> MLTSSSHHGRSYDVFLSFRGEDTRKTFVGHLFNALIEKGIHTFMDDKELKRGKSISSELMKAIGESRFAVVVFSKNYASSTWCLEELVKILEIHEKFELIVVPVFYDVDPSTVRKQNGEYAVCFTKFEANLVDDRDKVLRWREALTKVANISGHDLRNTYNGDESKCIQQILKDIFDKFCFSISITNRDLVGIESQIKKLSSLLRMDLKGVRLVGIWGMGGVGKTTAARALFNRYYQNFESACFLEDVKEYLQHHTLLYLQKTLLSKLLKVEFVDCTDTEEMCVILKRRLCSKKVLVVLDDVNHNDQLDKLVGAEDWFGSGSRIVITTRDMKLLKNHDVHETYEIKVLEKDEAIELFNLHAFKRSSPEKEFKELLNLVVDYTGGLPLALKVLGSLLYKEDLDVWISTIDRLKDNPEGEIMATLKISFDGLRDYEKSIFLDIACFFRGYNQRDMTALFHASGFHPVLGVKTLVEKSLIFILEDKIQMHDLMQEMGRQIAVQESPMRRIYRPEDVKDACIGDMRKEAIEGLLLTEPEQFEEGELEYMYSAEALKKTRRLRILVKEYYNRGFDEPVAYLPNSLLWLEWRNYSSNSFPSNFEPSKLVYLTMKGSSIIELWNGAKRLAFLTTLDLSYCHKLIQTPDFRMITNLERLILSSCDALVEVHPSVGFLKNLILLNMDHCISLERLPAIIQSECLEVLDLNYCFNLKMFPEVERNMTHLKKLDLTSTGIRELPASIEHLSSLENLQMHSCNQLVSLPSSIWRFRNLKISECEKLGSLPEIHGNSNCTRELILKLVSIKELPTSIGNLTSLNFLEICNCKTISSLSSSIWGLTSLTTLKLLDCRKLKNLPGIPNAINHLSGHGLQLLLTLEQPTIYERLDLLRIIDMSWCSCISSLPHNIWMLKFLRILCISYCSRLEYLPENLGHLEHLEELLADGTGILRLPSSVARLNKLEVLSFRKKFAIGPKVQYSSSMLNLPDDVFGSLGSLGSVVKLNLSGNGFCNLPETMNQLFCLEYLDITFCQRLEALPELPPSIKELYVDEHLALRIMEDLVIKCKELNLIAVTKIEYQNFYR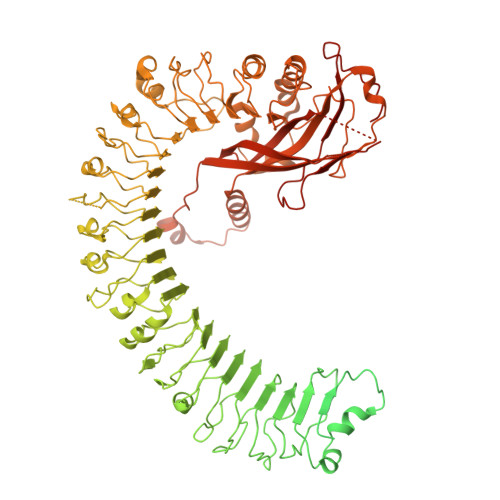WLDSIWSDVSELLENSQKQQLDDMLQLIPFSYLSTAKREEVLKIVIHGTRIPEWFRWQDRSATTMSVNLPEYWYTENFLGFAICCSCCFYHSARSYDVEFEGSMHHYNYDSSYWKEYEEPSYDFYERDSIEITAKLTPRHKGMRTEELKKVCSFSMNVLRRATAVPNMCFAFFPFNSLCHISNLQANNPNDYGIFETCLSPGDIRHRGKQWGFNLVYKDETGGSVTHEMLINRDYKDHDGDYKDHDIDYKDDDDK>MGSSHHHHHHSSSAALEVLFQGPMELFNRVGRVLKSQLTHWQQQQEAPEDLLERLLGEMELELIELRRALAQTIATFKSTERQRDAQQLIAQRWYEKAQAALDRGNEQLAREALGQRQSYQSHTEALGKSLGEQRALVEQVRGQLQKLERKYLELKSQKNLYLARLKSAIAAQKIEEIAGNLDNASASSLFERIETKILELEAERELLNPPPSPLDKKFEQWEEQQAVEATLAAMKARRSLPPPSS[60x]

The bacterial member PspA is part of the phage shock protein (psp) response that maintains structural integrity of membranes under stress conditions such as temperature and infection. The main effector of the Psp system is PspA, a 25 kDa protein consisting of six α-helices connected by short loops and an elongated hairpin, where the N-terminal helix α0 of the protein remains unfolded in the absence of membranes. Interestingly, PspA is related to eukaryotic and archaeal endosomal sorting complexes required for transport (ESCRT)-III proteins and has a similar structure. Here, we show that rods of bacterial ESCRT-III protein PspA internalize and thin membrane tubules by overcoming the required bending energy through progressive membrane binding of the N-terminal helix in the PspA assembly.

For our analyses, we refolded PspA in the presence of 50 nm sized small unilamellar EPL vesicles, similar to a recently described protocol. In the presence of EPL membranes, the rods had a wider diameter and a broader diameter distribution (200 to 345 Å) in comparison with the diameter values and distribution of the previously analyzed apo protein (180 to 290 Å). By segmenting the rods of the EPL-PspA sample and sorting the segments according to diameter through classification, we determined a total of 10 cryo-EM structures with resolutions ranging from 4.7 to 6.5 Å. While the imposed helical symmetry parameters suggested no architectural relationship between the PspA rods, helical lattice plots revealed that the left-handed helical rung corresponding to layer line ~110 Å in the power spectrum increased in Bessel order from n = 10, 11, 12…18 with increasing diameters of 200, 215, 235…345 Å, respectively. Upon insertion of an additional subunit into the helical rung, the assembly widens in discrete steps of around 20 Å up to a diameter of 345 Å. The rods with diameters larger than 280 Å were of particular interest as they showed enclosed double-layered lipid density in the cross-sectional top and side views in addition to the expected PspA protein densities, whereas rods of 270 Å diameter contained only partial lipid density and smaller diameters showed no density in the cross-section views. When comparing them with the previous apo structures, we observed that the structures of the EPL sample were identical to the apo structures with the same diameters, including their respective helical symmetry. The cryo-EM structures and MD simulations showed that only rods wider than 270 Å internalize and tubulate membranes. As indicated in the simulations, the energy required for membrane bending likely is too high for thinner rods to bend and internalize membrane tubules.> MDYEKTLLMPKTDFPMRGGLPNKEPQIQEKWDAEDQYHKALEKNKGNETFILHDGPPYANGNLHMGHALNKILKDFIVRYKTMQGFYAPYVPGWDTHGLPIEQALTKKGVDRKKMSTAEFREKCKEFALEQIELQKKDFRRLGVRGDFNDPYITLKPEYEAAQIRIF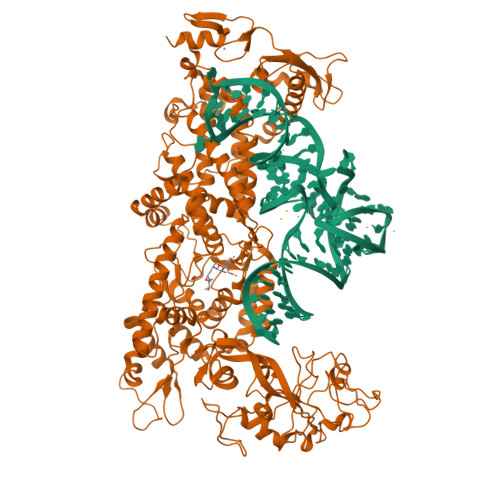GEMADKGLIYKGKKPVYWSPSSESSLAEAEIEYHDKRSASIYVAFNVKDDKGVVDADAKFIIWTTTPWTIPSNVAITVHPELKYGQYNVNGEKYIIAEALSDAVAEALDWDKASIKLEKEYTGKELEWVVAQHPFLDRESLVINGDHVTTDAGTGCVHTAPGHGEDDYIVGQQYELPVISPIDDKGVFTEEGGQFEGMFYDKANKAVTDLLTEKGALLKLDFITHSYPHDWRTKKPVIFRATPQWFASISKVRQDILDAIENTNFKVNWGKTRIYNMVRDRGEWVISRQRVWGVPLPVFYAENGEIIMTKETVNHVADLFAEHGSNIWFEREAKDLLPEGFTHPGSPNGTFTKETDIMDVWFDSGSSHRGVLETRPELSFPADMYLEGSDQYRGWFNSSITTSVATRGVSPYKFLLSHGFVMDGEGKKMSKSLGNVIVPDQVVKQKGADIARLWVSSTDYLADVRISDEILKQTSDDYRKIRNTLRFMLGNINDFNPDTDSIPESELLEVDRYLLNRLREFTASTINNYENFDYLNIYQEVQNFINVELSNFYLDYGKDILYIEQRDSHIRRSMQTVLYQILVDMTKLLAPILVHTAEEVWSHTPHVKEESVHLADMPKVVEVDQALLDKWRTFMNLRDDVNRALETARNEKVIGKSLEAKVTIASNDKFNASEFLTSFDALHQLFIVSQVKVVDKLDDQATAYEHGDIVIEHADGEKCERCWNYSEDLGAVDELTHLCPRCQQVVKSLV>[4x]SDAHHAHKGLNYGSFTKEHVLLTPKGYREWVFIGASVTPNELNDDKAAFPEFHNVYIDPTSWGHWKKTGEFRDGTVIVKELAGVGSKASPSGNGYFPGEFNGIQAMVKDSKRY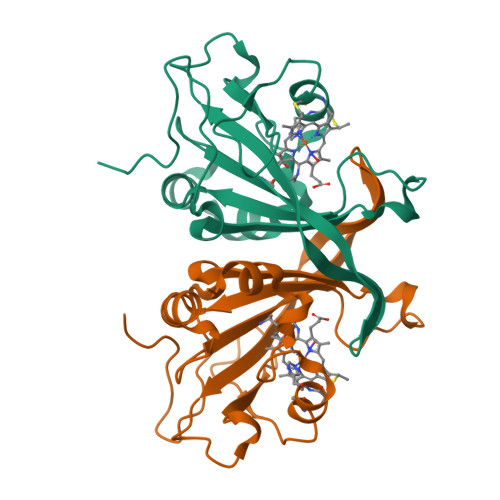PERPGNWAFFGFESYEAKQGIIQTDETCAACHKEHAAHDMVFTQFYPVLRAGKPSK>RLSLQNTAEIQHCLVNAGDVGCGVFECFENNSCEIRGLHGICMTFLHNAGKFDAQGKSFIKDALKCKAHALRHRFGCISRKCPAIREMVSQLQRECYLKHDLCAAAQENTRVIVEMIHFKDLLLHEPYVDLVNLLLTCGEEVKEAITHSVQVQCEQNWGSLCSILSFC[2x];>EARGATEEPSPPSRALYFSGRGEQLRLRADLELPRDAFTLQVWLRAEGGQRSPAVITGLYDKCSYISRDRGWVVGIHTISDQDNKDPRYFFSLKTDRARQVTTINAHRSYLPGQWVYLAATYDGQFMKLYVNGAQVATSGEQVGGIFSPLTQKCKVLMLGGSALNHNYRGYIEHFSLWKVARTQREILSDMETHGAHTALPQLLLQENWDNVKHAWSPMKDGSSPKVEFSNAHGFLLDTSLEPPLCGQTLCDNTEVIASYNQLSSFRQPKVVRYRVVNLYEDDHKNPTVTREQVDFQHHQLAEAFKQYNISWELDVLEVSNSSLRRRLILANCDISKIGDENCDPECNHTLTGHDGGDCRHLRHPAFVKKQHNGVCDMDCNYERFNFDGGECCDPEITNVTQTCFDPDSPHRAYLDVNELKNILKLDGSTHLNIFFAKSSEEELAGVATWPWDKEALMHLGGIVLNPSFYGMPGHTHTMIHQIGHSLGLYHVFRGISEIQSCSDPCMETEPSFETGDLCNDTNPAPKHKSCGDPGPGNDTCGFHSFFNTPYNNFMSYADDDCTDSFTPNQVARMHCYLDLVYQGWQPSRKPAPVALAPQVLGHTTDSVTLEWFPPIDGHFFERELGSACHLCLEGRILVQYASNASSPMPCSPSGHWSPREAEGHPDVEQPCKSSVRTWSPNSAVNPHTVPPACPEPQGCYLELEFLYPLVPESLTIWVTFVSTDWDSSGAVNDIKLLAVSGKNISLGPQNVFCDVPLTIRLWDVGEEVYGIQIYTLDEHLEIDAAMLTSTADTPLCLQCKPLKYKVVRDPPLQMDVASILHLNRKFVDMDLNLGSVYQYWVITISGTEESEPSPAVTYIHGSGYCGDGIIQKDQGEQCDDMNKINGDGCSLFCRQEVSFNCIDEPSRCYFHDGDGVCEEFEQKTSIKDCGVYTPQGFLDQWASNASVSHQDQQCPGWVIIGQPAASQVCRTKVIDLSEGISQHAWYPCTISYPYSQLAQTTFWLRAYFSQPMVAAAVIVHLVTDGTYYGDQKQETISVQLLDTKDQSHDLGLHVLSCRNNPLIIPVVHDLSQPFYHSQAVRVSFSSPLVAISGVALRSFDNFDPVTLSSCQRGETYSPAEQSCVHFACEKTDCPELAVENASLNCSSSDRYHGAQCTVSCRTGYVLQIRRDDELIKSQTGPSVTVTCTEGKWNKQVACEPVDCSIPDHHQVYAASFSCPEGTTFGSQCSFQCRHPAQLKGNNSLLTCMEDGLWSFPEALCELMCLAPPPVPNADLQTARCRENKHKVGSFCKYKCKPGYHVPGSSRKSKKRAFKTQCTQDGSWQEGACVPVTCDPPPPKFHGLYQCTNGFQFNSECRIKCEDSDASQGLGSNVIHCRKDGTWNGSFHVCQEMQGQCSVPNELNSNLKLQCPDGYAIGSECATSCLDHNSESIILPMNVTVRDIPHWLNPTRVERVVCTAGLKWYPHPALIHCVKGCEPFMGDNYCDAINNRAFCNYDGGDCCTSTVKTKKVTPFPMSCDLQGDCACRDPQAQEHS[2x]

Although first discovered as a placental antigen present in the circulation during human pregnancy, the metzincin metalloproteinase PAPP-A (pregnancy-associated plasma protein-A, pappalysin-1, EC 3.4.24.79) is ubiquitously expressed in human tissues. PAPP-A is able to cleave insulin-like growth factor binding proteins (IGFBP) -2, -4, and -5 in the extracellular environment. It consequently causes the release of bound bioactive IGF-1 or -2, which are potent growth factors. The paralogue proteins stanniocalcin (STC)-1 and -2 were recently identified as potent endogenous PAPP-A inhibitors and thus connected with the IGF system.

We find that the 2:2 PAPP-A·STC2 complex of ~500 kDa is a highly flexible structure with multiple contacts within and between the subunits. The 500 kDa 2:2 complex is composed of interacting homodimers, stabilized by many intra- and interchain disulfide bonds, several interdomain contacts, and several bound Ca2+ ions. Disulfide bonds link the two PAPP-A subunits and the two STC2 subunits, and a disulfide bond connecting each PAPP-A subunit with an STC2 subunit prevents dissociation of the complex. In particular, a specific disulfide bond between the subunits of STC2 and PAPP-A prevents dissociation, and interactions between STC2 and a module located in the very C-terminal end of the PAPP-A subunit prevent binding of its main substrate, IGFBP-4. Within the PAPP-A·STC2 complex, the C domains and the LNR3 modules of each PAPP-A subunit do not interact with the STC2 subunit to which the C120-C732 disulfide is formed, but rather the opposite subunit of the STC2 dimer. This reflects the crossing of the PAPP-A polypeptides at the PAPP-A dimerization disulfide, between M6 and SCR1. However, this truncated variant is also able to dimerize with a C-terminal variant starting at M5, and such heterodimers are active toward IGFBP-418. These data underscore that the M5 and M6 domains, here identified as responsible for formation of the dimerization interface, are sufficient for functional dimerization, and that the PAPP-A dimer has a trans configuration, which is maintained upon formation of the PAPP-A·STC2 complex. We demonstrate that IGFBP-4 has an overlapping binding site in the C domain, consequently defining this region as a substrate-binding exosite, and STC2 as an exosite inhibitor. While devoid of activity towards IGFBP-4, the active site cleft of the catalytic domain is accessible in the inhibited PAPP-A·STC2 complex, as shown by its ability to hydrolyze a synthetic peptide derived from IGFBP-4.> MRDYSELEIFEG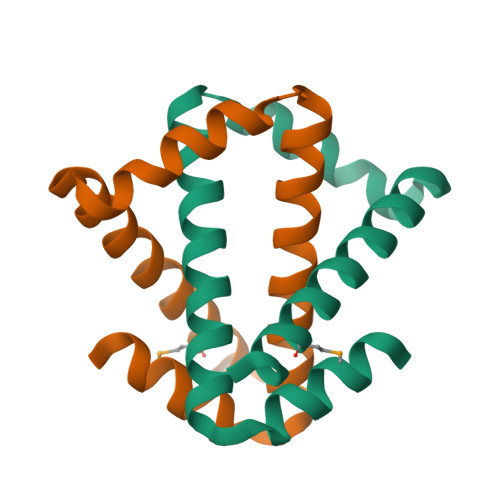NPLDKWNDIIFHASKKLSKKELERLLELLALLETFIEKEDLEEKFESFAKALRIDEELQQKIESRKTDIVIQSMANILSGNE> DDHSELLVNTKSGKVMGTRVPVLSSHISAFLGIPFAEPPVGNMRFRRPEPKKPWSGVWNASTYPNNCQQYVDEQFPGFSGSEMWNPNREMSEDCLYLNIWVPSPRPKSTTVMVWIYGGGFYSGSSTLDVYNGKYLAYTEEVVLVSLSYRVGAFGFLALHGSQEAPGNVGLLDQRMALQWVHDNIQFFGGDPKTVTIFGESAGGASVGMHILSPGSRDLFRRAILQSGSPNCPWASVSVAEGRRRAVELGRNLNCNLNSDEELIHCLREKKPQELIDVEWNVLPFDSIFRF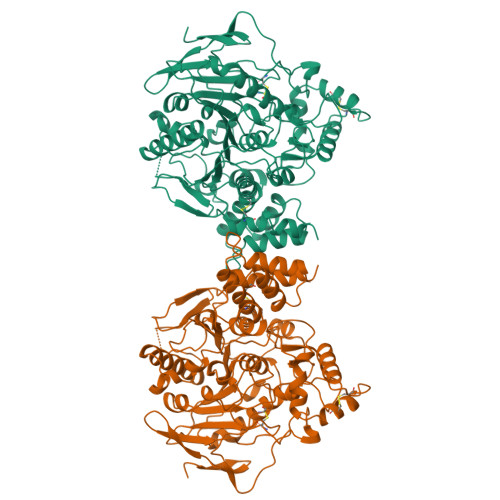SFVPVIDGEFFPTSLESMLNSGNFKKTQILLGVNKDEGSFFLLYGAPGFSKDSESKISREDFMSGVKLSVPHANDLGLDAVTLQYTDWMDDNNGIKNRDGLDDIVGDHNVICPLMHFVNKYTKFGNGTYLYFFNHRASNLVWPEWMGVIHGYEIEFVFGLPLVKELNYTAEEEALSRRIMHYWATFAKTGNPNEPHSQESKWPLFTTKEQKFIDLNTEPMKVHQRLRVQMCVFWNQFLPKLLNA>MQKA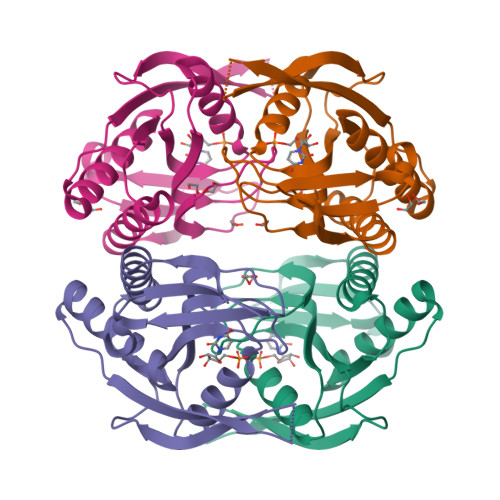VVMDEQAIRRALTRIAHEIIERNKGIDGCVLVGIKTRGIYLARRLAERIEQIEGASVPVGELDITLYRDDLTVKTDDHEPLVKGTNVPFPVTERNVILVDDVLFTGRTVRAAMDAVMDLGRPARIQLAVLVDRGHRELPIRADFVGKNVPTSRSELIVVELSEVDGIDQVSIHEK[2x]> GAEVGRLRYPPEMPGAEVKVYKKVDNVDLKLYIYKPADWKPADRRSAIVFFFGGGWQSGSPAQFRPQCEYFAGRGMVAMAADYRVGSRHNVKVADCVADAKSAIRWVRQHAAELGVDPQKIVASGGSAGGHLAACTVMVPDLEAPEEDHTISSQANAAILFNPVLILSREGLKDHVPRQDWEERLRERLGTEPKAVSPYHHIRAGLPPMIIFHGTADNTV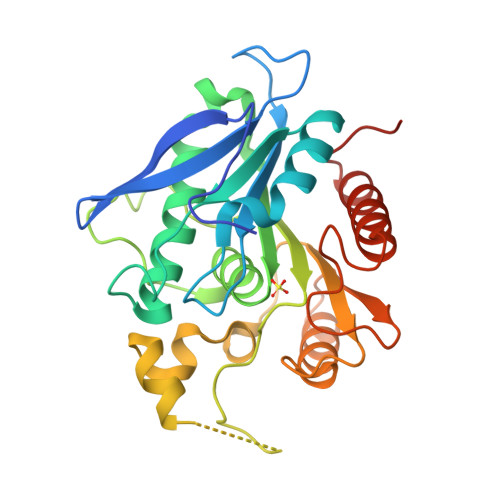PFETIRLFAEAMKKAGNRCELVPFEGAAHGFFNFGRGDNLAYQKTLELADEFLVEIGFLAPKGESQP>[4x]ETRPNHTIYINNLNEKIKKDELKKSLHAIFSRFGQILDILVSRSLKM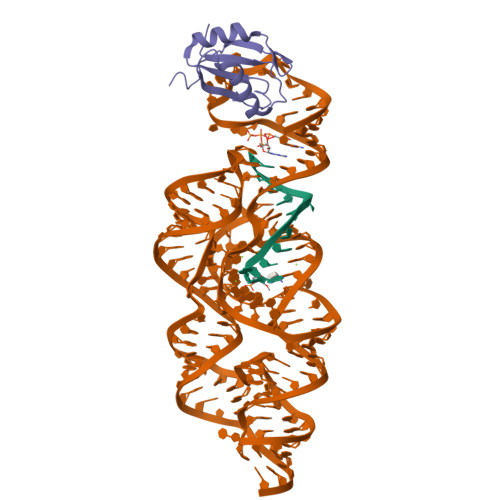RGQAFVIFKEVSSATNALRSMQGFPFYDKPMRIQYAKTDSDIIAKMK Here we identify the intracellular NAT16 as the human histidine acetyltransferase (HisAT) responsible for histidine acetylation in vitro and in vivo. Acetylhistidine is synthesized from histidine and acetyl coenzyme A (Ac-CoA) by a histidine acetyltransferase (HisAT, EC:2.3.1.33). We find that HisAT adopts a double-GNAT (Gcn5-related N-Acetyltransferase) fold where the N-terminal domain binds acetyl-CoA and with distinct active site conformation allowing the binding of histidine in between the two domains. Our results indicate that HisAT catalysis occurs via a ternary complex, and the ternary complex is likely stabilized by the oxyanion hole generated by the residues Gly123 and Leu124 of the β-bulge.

The HisAT crystals with CoA disulfide were obtained in the presence of histidine, arginine, and imidazole. In the structure where the buffer component imidazole was found in the active site, it was positioned in between Tyr74 and Trp246 in a similar way as the histidine side chain. This affinity probably explains the difference in enzyme activity between histidine and arginine, but not the poor quality of the other aromatic side chain amino acids as HisAT substrates. The HisAT crystals usually adopted the space group P63 where the packing seemed to be dependent on the crystal contact formed by the second CoA moiety of a CoA disulfide molecule, formed by two CoA molecules covalently linked by a disulfide bond between their thiol groups, at the active site. The crystals of the P63 space group invariably contained a CoA disulfide. The first CoA of the CoA disulfide bound to the canonical position and aligned well with the other molecules bound in this position except for the 3ʹ-AMP moiety that was poorly defined. The second CoA of the CoA disulfide was positioned in a cavity formed between the helices α3, α4, and the β-sheet segment composed of β5, β13, and β6.

> MKLESSETRPQEVEAEPRSGSGPEAEAEPLDFVVATEREFEEVLAISGGIYGGLDYLPSRYHSWLRDPDRTVVLAKRNGGVIALESVNVIDAGETVLVEGLRVAPWERGKGVAGLLQRFCSQLVKRQHPGVKVARLTRDDQLGPRELKKYRLITKQGILLVRFNASALLAGLGARLAALRTSGTFSPLPTEAVSEAGGDVARLLLSPSVQRDVLPGGTIIQDWQPYRPSESNLRLLAAKGLEWRVDSRARPRVLTLCTRPFPIPHGGDGTWRYLNIDAFGSDGAQVQSQLLWHLQRQAPRLVGLNVMCQLFLEPQLWSQLADFCQVGLGLELVKGYTEQYLLEADIHHHHHH> GSMLSAFTARPIIELKPRDKSRIECILAYGD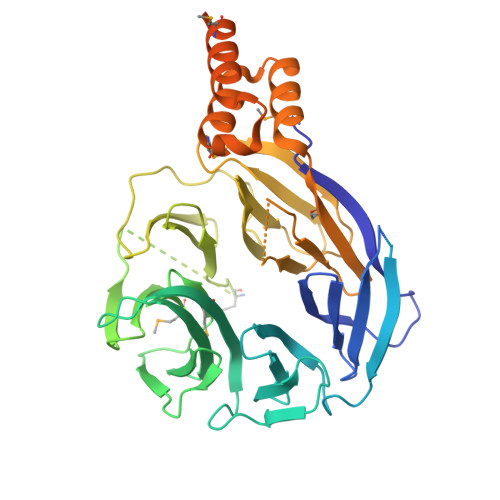RVLVGLNTGSLRVYRVNDLSPSPSPANPSDSQSPEASQSSVNPDPSSSTQDPSSQPDSQPVVPQQKPTDLLREIERFSPRAIEQLAIIKEANTLVSLSNYCVSLHDLHTFEPIASPLPRTKNASGFAVTSNIVKDPATGIPEIISRLAVSVKRRLLLWSWHESELEEEVKEVVLTESIRSMTWACATRLVCGMNSGFVVVDVETGTVEDILGPPGGAAGGNQGRWGAVSAGGMGYMGLGGYMPKPLCTKLADGQLLLAKDVNTLFIDDTGKALEKRQIPWQAAPDGIGYSYPYILALQPPAKGCLEVRNPDTLSLLQTLSLPGAAALHFPPPTVSLAHAGKGFHVLSDRVVWKMDATDYDSQVEELVRGGKLDEAISVLTMLEDALLKNKTETLREVKMQKAEVLFRQKKYRESMDLFNEDEVNAPPERVLRLFPKSIAGELSGVEEEKQGQSQQSDSEQEGSSNGTATAD> HHHSSGRENLYFQGMHIAIIGAAGMVGRKLTQRLVKDGSLGGKPVEKFTLIDVFQPEAPAGFSGAVDARAADLSAPGEAEKLVEARPDVIFHLAAIVSGEAELDFDKGYRINLDGTRYLFDAIRIANGKDGYKPRVVFTSSIAVFGAPLPYPIPDEFHTTPLTSYGTQKAICELLLSDYSRRGFFDGIGIRLPTICIRPGKPNAAASGFFSNILREPLVGQEAVLPVPESIRHWHASPRSAVGFLIHGAMIDVEKVGP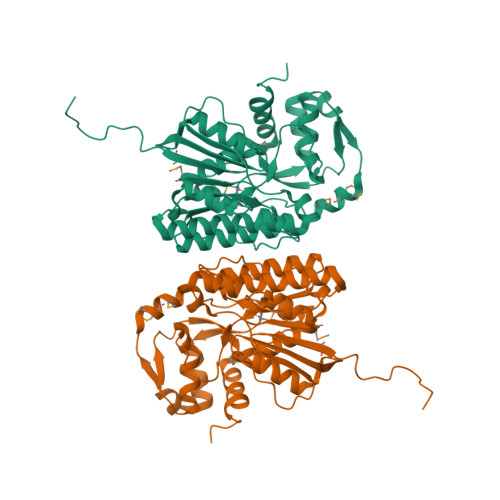RRNLSMPGLSATVGEQIEALRKVAGEKAVALIRREPNEMIMRMCEGWAPGFEAKRARELGFTAESSFEEIIQVHIEDELGGSLK Bacillus subtilis expresses TasA (translocation-dependent antimicrobial spore component) as the major biofilm protein, which aided by TapA (TasA anchoring/assembly protein, YqxM) can convert into stable oligomeric structures to form the biofilm matrix. In summary, TapA consists of an Ig domain in its core and flexible N and C termini. TapA thus functions as a chaperone in analogy to the chaperone-usher pathway since it already has a complete and especially stable V-set Ig fold and has the ability to complement TasA in the process of filament formation by donating its previously unstructured N-terminal strand. Owing to the stability of the TapA Ig domain, it is not able to open a cleft to receive a donor strand, and thus can only be located at the beginning of a filament, acting as filament inducer.

The relevance of different TapA sections for promoting oligomer formation was investigated by using truncated proteins. Deleting the N terminus resulted in TapA75-190 that yielded only negligible amounts of oligomers in an AUC run with equimolar concentrations (Fig. 2C, turquoise curve; orange curve for comparison). In agreement with the AUC experiments, the addition of 50 µM TapA75-190 to 250 µM TasA does not lead to a reduction of folded TasA (blue curve), supporting the notion that the N-terminal residues of TapA are critical for stimulating oligomerization. The additional hydrogen bonding suggests a higher stability of TapA71-190, which is supported by the TSA data (Tm = 60 °C for TapA71-190 and 46 °C for TapA75-190). Structural integrity is supported by a disulfide bond linking C92 and C188. Constructs with odd numbers of cysteines such as TapA60-190 and TapA66-190 showed a tendency to form dimers via disulfide bond formation with their free cysteine C68. TapA44-253, TapA54-190, and TapA75-190, on the other hand, appeared as monomers, since they contain even numbers of cysteines.

> DQSDLHISDQTDTKGTVCSPFALFAVLENTGEKLKKSKWKWELHKLENARKPLKDGNVIEKGFVSNQIGDSLYKIETKKKMKPGIYAFKVYKPAGYPANGSTFEWSEPMRLAKCDE> GAGACCTGTA;> CGGACAGTGCA;> TCTGCACTGTGG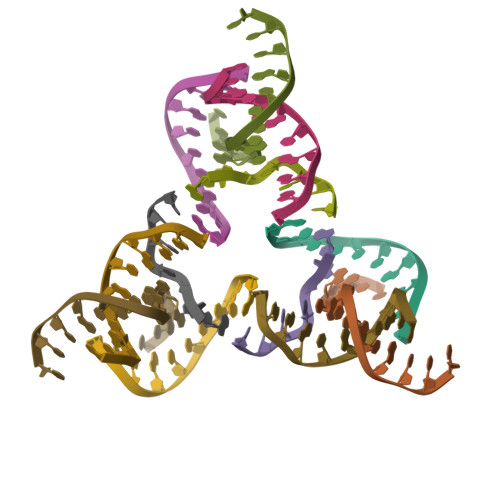TC;> ACACCGT>GHMGKPDISAKDLRNIMYDHLPGFGTAFHQLVQVICKLGKDSNSLDIIHAEFQASLA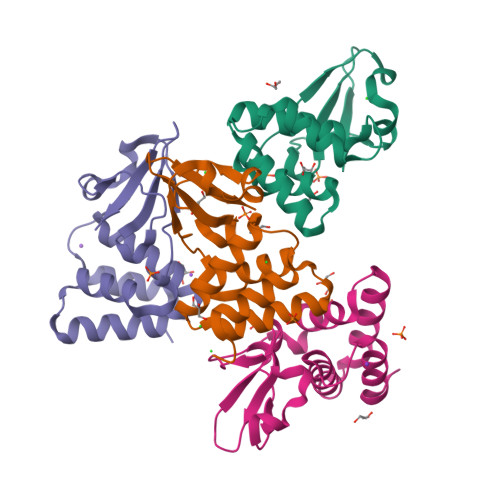EGDSPQCALIQITKRVPIFQDAAPPVIHIRSRGDIPRACQKSLAPVPPSPKIDRGWVCVFQLQDGKTLGLKI[4x]> MAALRNGLEGSSEETSFHDESLQDDREEIENNSYHMHPAGIILTKVGYYTIPSMDDLAKITNEKGECIVSDFTIGRKGYGSIYFEGDVNLTNLNLDDIVHIRRKEVVVYLDDNQKPPVGEGLNRKAEVTLDGVWPTDKTSRCLIKSPDRLADINYEGRLEAVSR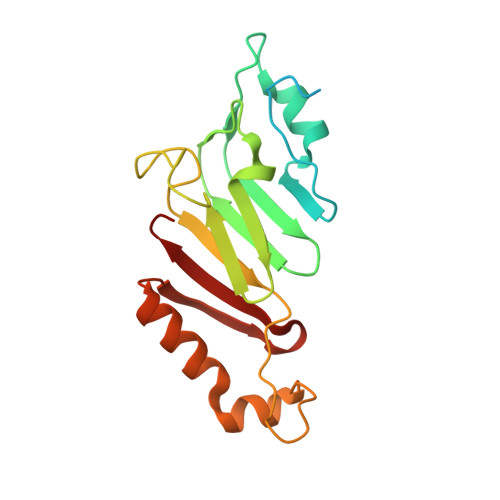KQGAQFKEYRPETGSWVFKVSHF>[4x]MGHHHHHHAMEGKITPVSVKKVDDKVTLYKTTATADSDKFKISQILTFNFIKDKSYDKDTLVLKATGNINSGFVKPNPNDYDFSKLYWGAKYNVSISSQSNDSVNVVDYAPKNQNEEFQVQNTLGYTFGGDISISNGLSGGLNGNTAFSETINYKQESYRTTLSRNTNYKNVGWGVEAHKIMNNGWGPYGRDSFHPTYGNELFLA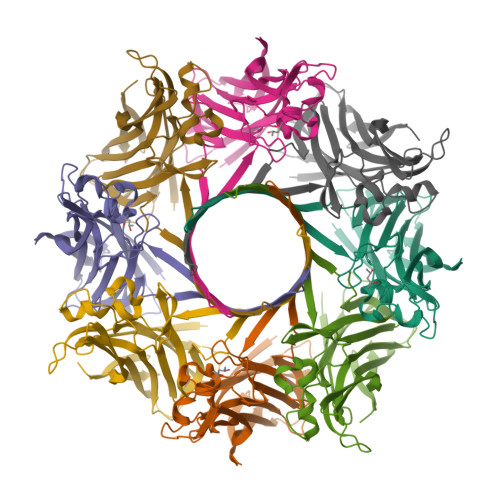GRQSSAYAGQNFIAQHQMPLLSRSNFNPEFLSVLSHRQDGAKKSKITVTYQREMDLYQICWNGFYWAGANYKNFKTRTFKSTYEIDWENHKVKLLDTKETENNK;>[4x]MGHHHHHHAMENKIEDIGQGAEIIKRTQDITSKRLAITQNIQFDFVKDKKYNKDALVVKMQGFISSRTTYSDLKKYPYIKRMIWPFQYNISLKTKDSNVDLINYLPKNKIDSADVSQKLGYNIGGNFQSAPSIGGSGSFNYSKTISYNQKNYVTEVESQNSKGVKWGVKANSFVTPNGQVSAYDQYLFAQDPTGPAARDYFVPDNQLPPLIQSGFNPSFITTLSHERGKGDKSEFEITYGRNMDATYAYVTRHRLAVDRKHDAFKNRNVTVKYEVNWKTHEVKIKSITPK> VPAPGETRACGRKL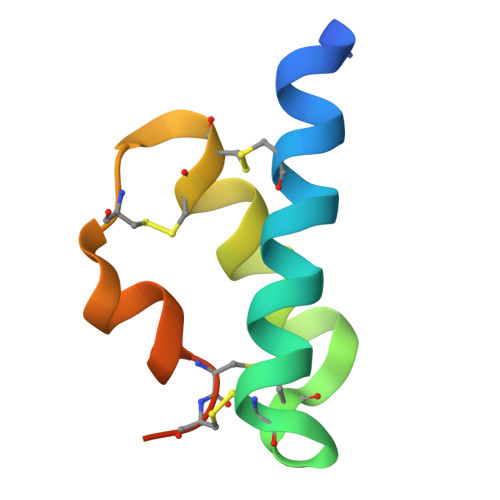ISLVMAVCGDLCNPQEGKDIATECCGNQCSDDYIRSACCPHHHHHH>MTKPLDGINVLDFTHVQAGPACTQMMGFLGANVIKIERRGSGDMTRGQLQDKPNVDSLYFTMFNCNKRSIELDMKTPEGKELLEQMIKKADVMVENFGPGALDRMGFTWEYIQELNPRVILASVKGYAEGHANEHLKVYENVAQCSGGAAATTGFWDGPPTVSGAALGDSNSGMHLMIGILAALEIRHKTGRGQKVAVAMQDAVLNLVRIKLRDQQRLERTGILAEYPQAQPNFAFDRDGNPLSFDNITSVPRGGNA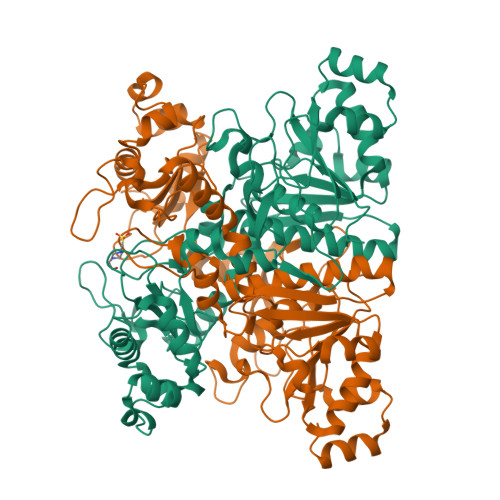GGGGQPGWMLKCKGWETDADSYVYFTIAANMWPQICDMIDKPEWKDDPAYNTFEGRVDKLMDIFSFIETKFADKDKFEVTEWAAQYGIPCGPVMSMKELAHDPSLQKVGTVVEVVDEIRGNHLTVGAPFKFSGFQPEITRAPLLGEHTDEVLKELGLDDAKIKELHAKQVV[4x]> QRLPLSKLVLTGERHYTRNDDIRQSILALGEPGTFMTQDVNIIQTQIEQRLPWIKQVSVRKQWPDELKIHLVEYVPIARWNDQHMVDAEGNTFSVPPERTSKQVLPMLYGPEGSANEVLQGYREMGQMLAKDRFTLKEAAMTARRSWQLTLNNDIKLNLGRGDTMKRLARFVEL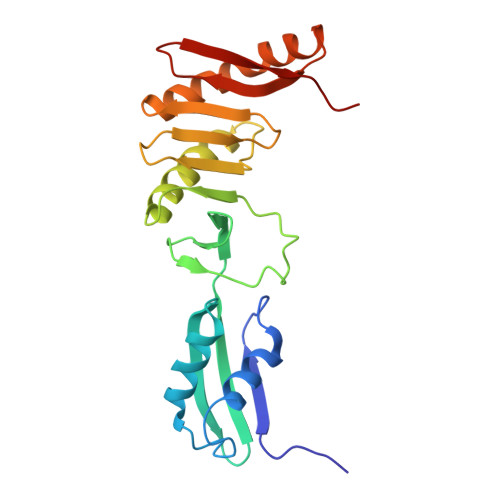YPVLQQQAQTDGKRISYVDLRYDSGAAVGWAPLPP> GGMQADKCPVTGATATTARGDSVEFDFFAAPQAYRRVAAEHRADGAFHSSRGDSFWVLSTYEGICAAFRDEDTFSVSRVSAADGAEDERWIPLTIQGRTHNEWRRRLAAWFTPQRARDLTPAIRANARRRISAFVDRGEVSFSDEFARPYVLENLMLAVGWPLADLDHLLA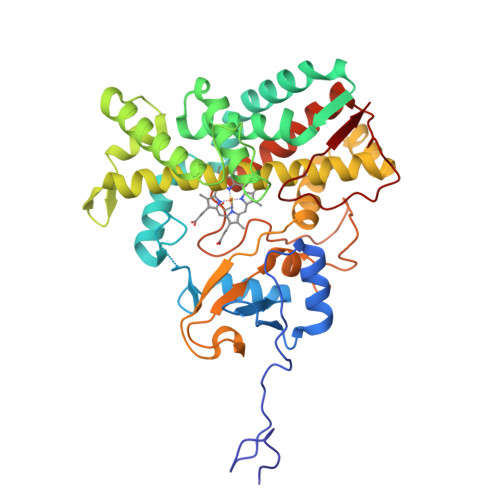INVAMIRSREAPDPRQAFNAETAFPALQEYVRRHVARRRAEPVEGDLTSATFDWEIDGTPVSDADRESLLTVLFLAGVDSTVNHMANGIQHLAHHPGDRHRFLRDPEVRPAAVEEFLRVNSCMYPGRLATREGAGGVASQGDTVLLPLALANYDPAVFPEPERVDFDREQNPHIAFGTGHHQCLGAAYARAQILTAWEEWHELIPDYRLPDPTVEPPFLRNVYDLRIVW;> GGMQADKCPVTGATATTARGDSVEFDFFAAPQAYRRVAAEHARDGAFHSSRGDSFWVLSTYEGICAAFRDEDTFSVSRVSAADGAEDERWIPLTIQGRTHNEWRRRLAAWFTPQRARDLTPAIRANARRRISAFVDRGEVSFSDEFARPYVLENLMLAVGWPLADLDHLLAINVAMIRSREAPDPRQAFNAETAFPALQEYVRRHVARRRAEPVEGDLTSATFDWEIDGTPVSDADRESLLTVLFLAGVDSTVNHMANGIQHLAHHPGDRHRFLRDPEVRPAAVEEFLRVNSCMYPGRLATREGAGGVASQGDTVLLPLALANYDPAVFPEPERVDFDREQNPHIAFGTGHHQCLGAAYARAQILTAWEEWHELIPDYRLPDPTVEPPFLRNVYDLRIVW> MIGMDRRSGLPLSGLAHLKQSVEDIL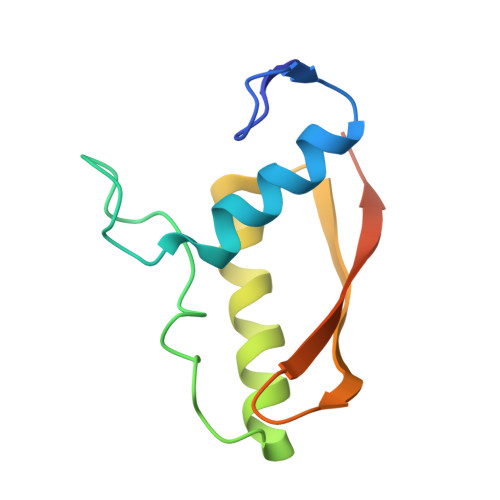TTPLGSRRMRPEYGSKLRRMVDMPVSEGWKSAVQAEVARSLGRWEPRIGLSAVRVVAVVDGRVDLLLSGVFEGENINMEVSA> MDPGTVLEISRSLKKRMQ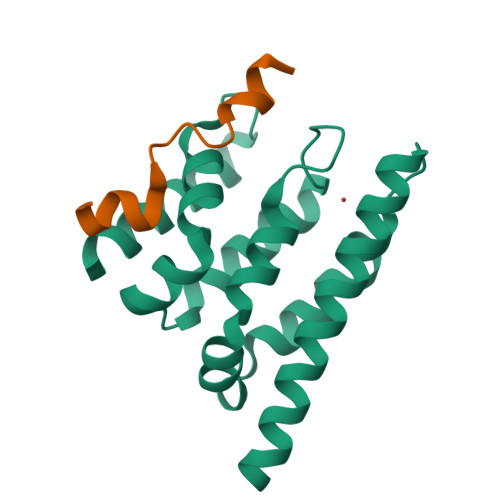DILKKDNANNLEGRPATGKIENVEEISDILMSKALQESLLDEGILDEIKGWLEPLPDKSMPNIKIRKRLLDVLKTMKIHKEHLVTSGVGKIVYFYSINPKESKEVRASAKALVQKWTNEVFKPEGGD;> GSHMFFEIFGTGEEYRYVLESDP>DNSYKMDYPEMGLCIIINNKNFHKS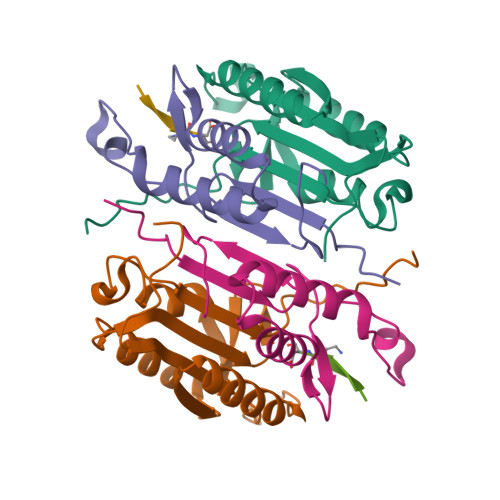TGMTSRSGTDVDAANLRETFRNLKYEVRNKNDLTREEIVELMRDVSKEDHSKRSSFVCVLLSHGEEGIIFGTNGPVDLKKITNFFRGDRCRSLTGKPKLFIIQACRGTELDCGIET[2x];>[2x]CHKIPVEADFLYAYSTAPGYYSWRNSKDGSWFIQSLCAMLKQYADKLEFMHILTRVNRKVATEFESFSFDATFHAKKQIPCIVSMLTKELYFYHH;>[2x]XITVAD>[2x]QAGFDLLNDGRPETLWLGIGTLLMLIGTFYFIARGWGVTDKEAREYY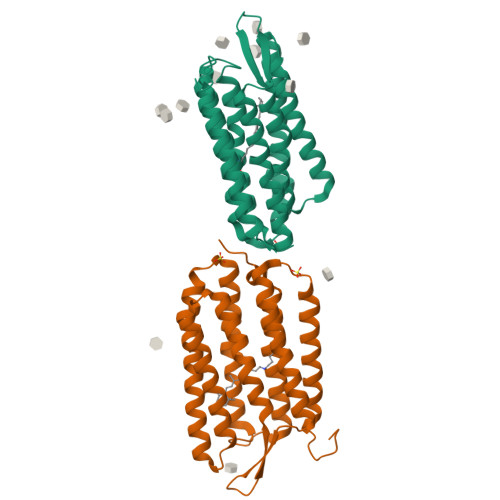AITILVPGIASAAYLAMFFGIGVTEVELASGTVLDIYYARYADWLFTTPLLLLDLALLAKVDRVTIGTLIGVDALMIVTGLIGALSKTPLARYTWWLFSTIAFLFVLYYLLTSLRSAAAKRSEEVRSTFNTLTALVAVLWTAYPILWIVGTEGAGVVGLGIETLAFMVLDVTAKVGFGFVLLRSRAILGETEAPEPSAGADASAAD> GPLGSMASTNAESQLQRIIRDLQDAVTELSKEFQEAGEPITDDSTSLHKFSYKLEYLLQFDQKEKATLLGNKKDYWDYFCACLAKVKGANDGIRFVKSISELRTSLGKGRAFIRYSLVHQRLADTLQQCFMNTKVTSDWYYARSPFLQPKLSSDIVGQLYELTEVQFDLASRGFDLDAAW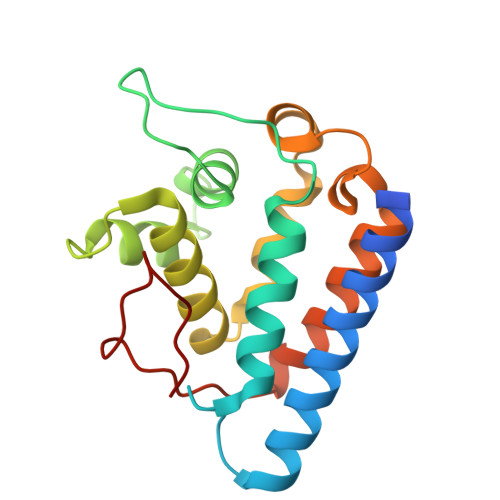PTF> AWPKVQPEVNIGVVGHVDHGKTTLVQAITGIWTSKHSEELKRGMTIKLGYAETN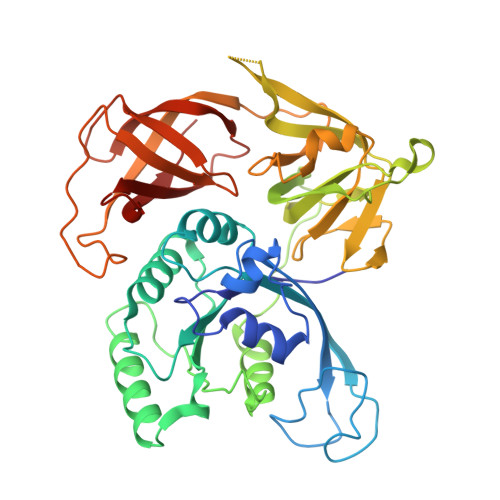IGVCESCKKPEAYVTEPSCKSCGSDDEPKFLRRISFIDAPGHEVLMATMLSGAALMDGAILVVAANEPFPQPQTREHFVALGIIGVKNLIIVQNKVDVVSKEEALSQYRQIKQFTKGTWAENVPIIPVSALHKINIDSLIEGIEEYIKTPYRDLSQKPVMLVIRSFDVNKPGTQFNELKGGVIGGSIIQGLFKVDQEIKVLPGLRVEKQGKVSYEPIFTKISSIRFGDEEFKEAKPGGLVAIGTYLDPSLTKADNLLGSIITLADAEVPVLWNIRIKYNLLERVVGAKEMLKVDPIRAKETLMLSVGSSTTLGIVTSVKKDEIEVELRRPVAVWSNNIRTVISRQIAGRWRMIGWGLVEI>[2x]IVGGYNCEENSVPYQVSLNSGYHFCGGSLINEQWV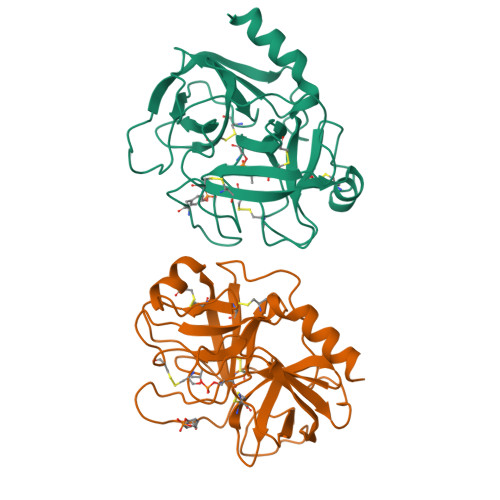VSAGHCYKSRIQVRLGEHNIEVLEGNEQFINAAKIIRHPQYDRKTLNNDIMLIKLSSRAVINARVSTISLPTAPPATGTKCLISGWGNTASSGADYPDELQCLDAPVLSQAKCEASYPGKITSNMFCVGFLEGGKDSCQGDSGGPVVCNGQLQGVVSWGDGCAQKNKPGVYTKVYNYVKWIKNTIAANS[({[3-chloro-4-(1H-tetrazol-5-yl)phenyl]sulfonyl}amino)methyl]boronic acid | C8 H9 B Cl N5 O4 S | 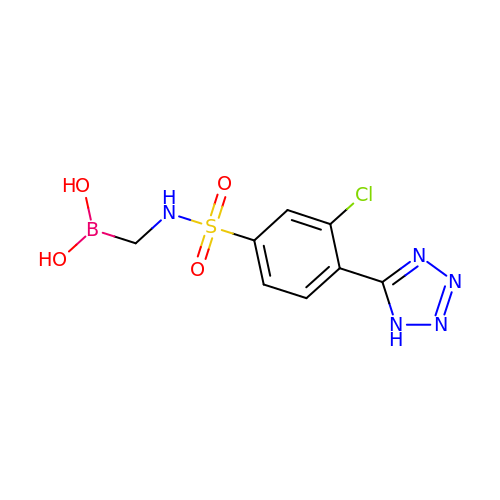PFJLILKXTJECEF-UHFFFAOYSA-N>GPDSITEYPDKTIHQLFTEQVEKTPEHVAVVFEDEKVTYRELHERSNQLARFLREKGVKKESIIGIMMERSVEMIVGILGILKAGGAFVPIDPEYPKERIGYMLDSVRLVLTQRHLKDKFAFTKETIVIEDPSISHELTEEIDYINESEDLFYIIYTSGTTGKPKGVMLEHKNIVNLLHFTFEKTNINFSDKVLQYTTCSFDVCYQEIFSTLLSGGQLYLIRKETQRDVEQLFDLVKRENIEVLSFPVAFLKFIFNEREFINRFPTCVKHIITAGEQLVVNNEFKRYLHEHNVHLHNHYGPSETHVVTTYTINPEAEIPELPPIGKPISNTWIYILDQEQQLQPQGIVGELYISGANVGRG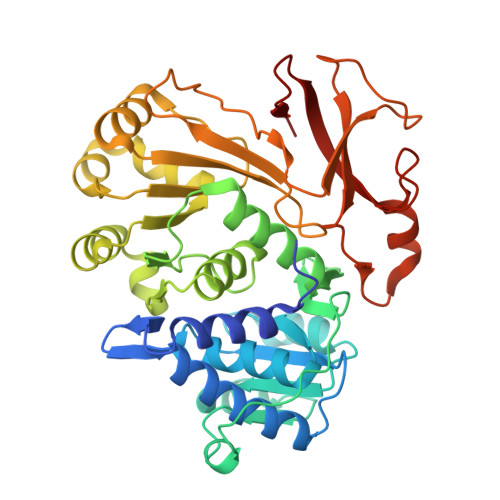YLNNQELTAEKFFADPFRPNERMYRTGDLARWLPDGNIEFLGRA[4x]>GMSSDVQKGDNLETPGARDLLLQTASNIMREGDVVDISLSELSLRSGLNSALVKYYFGNKAGLLKALLDRDMENIVKSVDALLAKDDMSPEAKLRRHISKCIDTYYDYPYLNRLLMRLVRDSDEAEAKRIADQYLLPLHRAYNRFIGEGVKAGVFRPINPQLFYF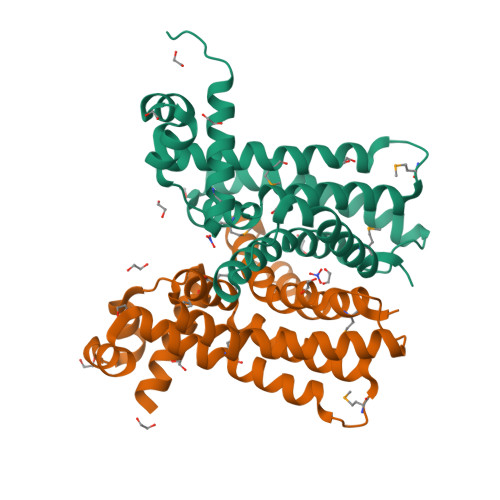TVTGAADRFFSARLVLKHCFDQDTLTEQLRDSYREHTVDFIMAGILAH[4x]>[2x]GSHMASSCAVQVKLELGHRAQVRKKPTVEGFTHDWMVFVRGPEHSNIQHFVEKVVFHLHESFPRPKRVCKDPPYKVEESGWAGFILPIEVYFKNKEEPRKVRFDYDLFLHLEGHPPVNHLRCEKLTFNNPTEDFRRKLLKA;>QTARXSSTGG[2x]

One of the major and widespread PTMs is acylation of the ε-amino group of lysine residues. Canonical acyllysine readers, bromodomain and double PHD finger (DPF), display comparable binding capabilities toward various short acyl chain modifications, and while the YEATS domain exhibits preference for crotonyllysine, it still associates albeit more weakly with other acyllysine marks. In this study, we elucidate the significance of π stacking components in targeting of acetyllysines by the YEATS domains and report a previously uncharacterized DNA-binding activity of the human AF9-YEATS domain. Collectively, our results have illuminated the mechanistic basis underlying distinct recognition of acyllysine PTMs by the YEATS domains of yeast Taf14 and human AF9, allowing us to develop a Taf14-YEATS module that selects for the crotonyl modification and discriminates against saturated acyl modifications.

We next explored the possibility of engineering an AF9-based acyllysine-specific reader through mutating Y78 in AF9-YEATS to a tryptophan and therefore re-creating the WA motif seen in the Taf14-YEATS G82A mutant. Although NMR titration experiments revealed a tight interaction of AF9-YEATS Y78W with H3K9cr, binding affinities measured by fluorescence spectroscopy indicated that this mutant does not differentiate between H3K9cr and H3K9ac and associates with both peptides with a Kd of 2 μM. To explain the different behavior of Taf14-YEATS G82A and AF9-YEATS Y78W, we obtained the crystal structure of AF9-YEATS Y78W in complex with H3K9cr peptide. In this complex, W78 was in a single r1 conformation, which was engaged in π stacking with the crotonyl amide. Notably, A79 imposed steric hindrance on W78 to a higher degree than on wild-type Y78 at this position, resulting in a tilted conformation of W78. W78 is incapable of adopting the r2 conformation necessary for π stacking with the alkene group most likely because of steric hindrance from F28. Additional mutation of A79 to a glycine in AF9, to recapitulate the Taf14’ WG motif, failed to induce the selectivity as the AF9-YEATS Y78WA79G mutant bound equally well to either H3K9cr or H3K9ac peptide.> MLPKPGTYYLPWEVSAGQVPDGSTLRTFGRLCLYDMIQSRVTLMAQHGSDQHQVLVCTKLVEPFHAQVGSLYIVLGELQHQQDRGSVVKA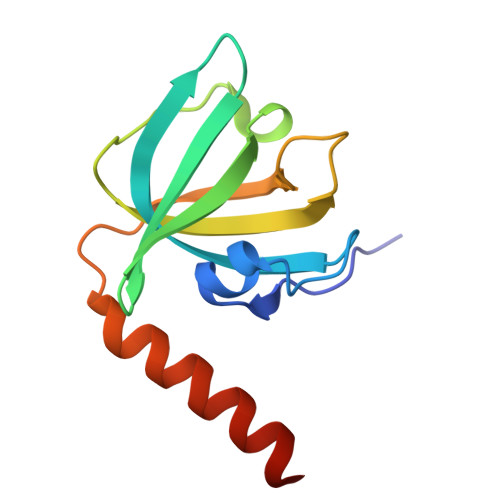RVLTCVEGMNLPLLEQAIREQRLYKQERGGSQ> MSEIILTPKEQPEVPLEAPNIKPDVFAGKSIEEIKNIQIMHGNEVVKLGDFFEVSG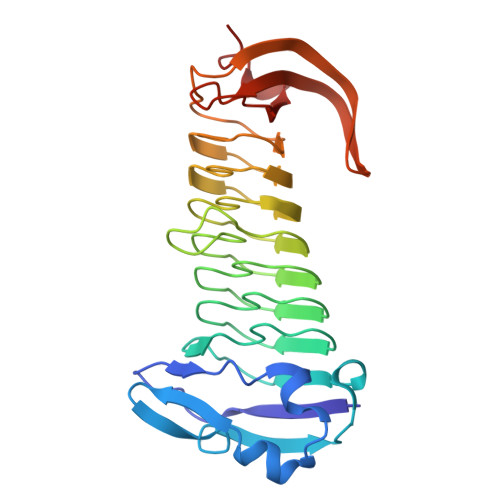EPADAPEDIKIIIDGDVYNTKRIGQEMTAGEIIVRGNVNMYVGAGMKGGKITVEGNAGSWAGQDMRGGEIEILGDAGDYVGSSYRGDWRGMSGGTITVHGNADNEIGEYMNGGKIIIKGDVNIMPGIHMNNGLIIIEGNVVARAGGEMAGGTIVVKGMMQEFLAGFKYLGVEKDIEVDGEELPGAFYKFEGDHAIKGAKGIVYAAVGCNGHIAP The envelope of Gram-negative pathogens, such as Acinetobacter baumannii and Pseudomonas aeruginosa, contains unique tripartite machineries that export noxious compounds from the cell. MacA-MacB-TolC contains similar components as the relatively well-characterized tripartite RND transporters AcrA-AcrB-TolC in E. coli and MexA-MexB-OprM in P. aeruginosa. However, the ABC protein MacB is unrelated to AcrB and MexB, which form large trimeric complexes in the plasma membrane, raising questions about the structure and domain organization of MacB in the tripartite efflux pump. Here, we present the crystal structure of MacB, and show that, by analogy to RND transporters, the MacB homodimer contains two large periplasmic domains (PLDs) that enable the interactions with the other components in this tripartite efflux pump.

MacB was purified and its crystal structure was solved at 3.4-Å resolution. A non-critical polypeptide segment between position 248 and 259 at the exterior of the NBD was found to be disordered. Two MacB monomers have a biological twofold rotation axis at the centre of the dimer. Each monomer in the dimer has essentially an identical structure (~1.1-Å RMSD in Cα position), and has elongated TMs (TM1 and TM2) protruding about 25 Å at the periplasmic side of the phospholipid bilayer. The interface between the monomers in the MacB dimer is extensive (2188.9 Å2) with major contributions from the TMDs (1053.0 Å2, 48%), PLDs (676.1 Å2, 31%) and NBDs (417.0 Å2, 19%). The TMD of MacB encompasses four TMs per monomer, which is the smallest number among currently characterized ABC exporters. The TMs are not swapped between the half-transporters and lack the helical extensions into intracellular domains as found in most type-I ABC exporters. Even though the MacB monomer has only one cytoplasmic loop, MacB preserves two CHs as observed in other ABC exporters. CH1 is present in the intracellular loop between TM2 and TM3, whereas CH2 is located in the carboxy terminus of MacB. Unlike Sav1866 and MsbA, in which CH1 contacts the NBDs of respective monomers and CH2 interacts with the NBD of the opposite monomer exclusively, the two CHs in MacB only contact one NBD within the same monomer.

>MHHHHHHMTKQALLEVSNLVREFPAGESTIQILKGIDLTIYEGELVAIVGQSGSGKSTLMNILGCLDRPTSGSYKVNGQETGKLEPDQLAQLRREYFGFIFQRYHLLGDLSAEGNVEVPAVYAGVTPADRKQRATALLTELGLGTKTQNRPSQLSGGQQQRVSIARALMNGGDVILADEPTGALDSHSGVEVMRILRELNAAGHTIILVTHDMQVAKNATRIIEISDGEIISDRPNVPDQSLEEVKSDPDAAPALQNKQKKGKSISAWRSTLDRLSEAFQMALLSMNAHRMRTFLTMLGIIIGIASVVTVVALGNGSQQQILSNISSLGTNTITVFQGRGFGDNSKTANFKTLVPADADALMTQPYVSAVSPMVSTSKTMRYQQNEANATINGVSNDYFDVKGLVFKDGQTFDQRSVRDRSQDVVIDTNTQKQFFSDGTNPIGQVVLLGSVPARIIGIVEPQTSGMGSDDTLNVYMPYTTVMSRMLGQAHVRNIVVRINDKYSTSAAENAIVNLLTQRHGAQDIFTMNSDSIRQTIEKTTSTMTLLVSAIAVISLVVGGIGVMNIMLVSVTERTQEIGVRMAVGARQSDILQQFLIEAILVCLIGGVLGVLLSLGLGQLINKFAGGNFAVAYSTTSIVAAFVCSTLIGVVFGFLPAKNAAKLDPVAALSRE[2x]> GHMSSKIFKNCVIYINGYTKPGRLQLHEMIVLHGGKFLHYLSSKKTVTHIVASNLPLKKRIEFANYKVVSPDWIV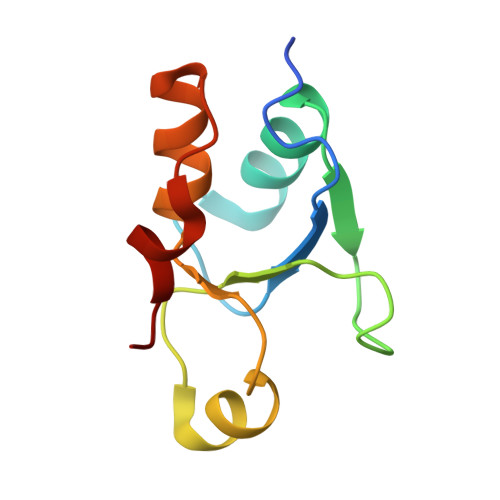DSVKEARLLPWQNYSLTS N-(2-phenylethyl)adenosine | C18 H21 N5 O4 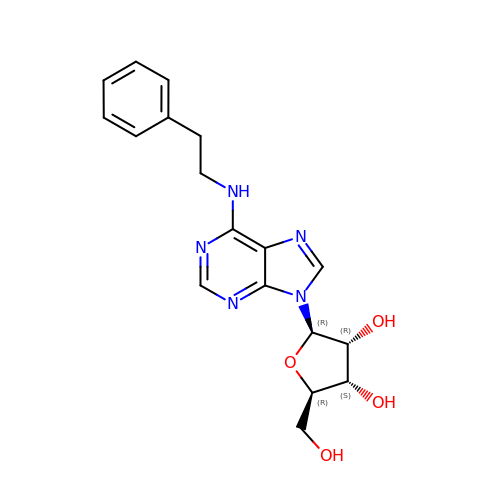| LGZYEDZSPHLISU-SCFUHWHPSA-N> MADVAGTSNRDFAGREQRLFNSEQYNYNNSLNGEVSVWVYAYYSDGSVLVINKNSQYKVGISETFKALKEYRCGQHNDSYDECEVNQSIYYPNGGDARKFHSNAKPRAIQIIFSPSVNVRTIKMAKGNAVSVPDEYLQRSHPWEATGIKYRKIKRDGEIVGYSHYFELPHEYNSISLAVSGVHKNPSSYNVGCCHNVMDVFQSCDL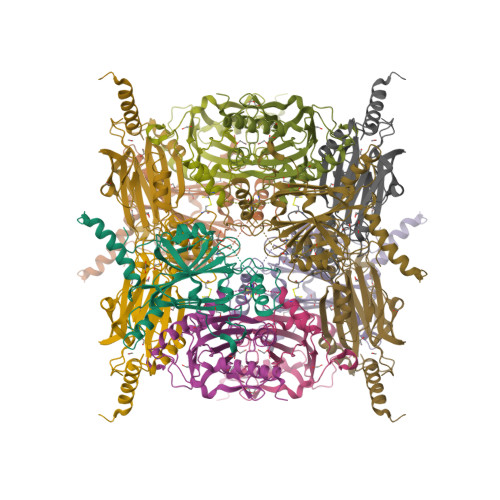ALRFCNRYWAELELVNHYISPNAYPYLDINNHSYGVALSNRQ4-(1H-pyrrol-1-yl)pyridine-2-carboxylic acid | C10 H8 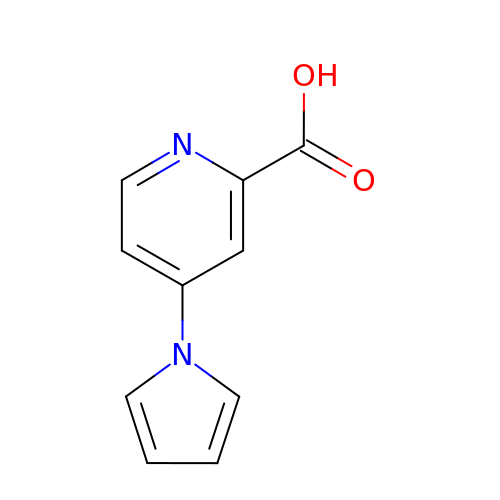N2 O2 | WGDPWMLPQRTMBY-UHFFFAOYSA-N To provide a molecular basis for designing better drugs targeting polymerases, African swine fever virus DNA Polymerase X (Pol X) was used as a model for the study. As the simplest DNA polymerase identified to date, Pol X belongs to the polymerase X family and is constituted of 174 amino acids. In this chemical reaction, metal-ion A (MeA) is a catalytic ion and decreases the pKa of 3′-OH, facilitating its attack on the α-phosphate of the incoming dNTP, and metal-ion B (MeB) stabilizes the dNTP-DNA-polymerase complex and increases the electrophilicity of the phosphorus center. To clearly understand the phosphodiester-bond-formation mechanism and the metal-ion catalysis of polymerases, we designed modified dNTP substrates with a chiral α-phosphorus center (α-P center) using a single selenium atom, without affecting the overall and local structures, to explore the absolute configuration inversion and probe the mechanisms of the metal ion–oxygen interactions.

To capture the reaction at the post-polymerization state, we designed and applied the crystallization droplets containing dGTPαSe-Rp, DNA-II, and Pol X. Surprisingly, we found that in one asymmetric unit, there was one substrate complex and three product complexes, including two DNA duplexes with four enzyme molecules. In other words, in the unit cell, the phosphoryl transfer reaction took place in three product complexes, whereas the last one was trapped in a transition-like state, where the incoming dGTPαSe-Rp paired with 5′-dC of the template strand. In the substrate complex, though two Me2+ ions at the active center coordinated with the incoming dGTPαSe-Rp, the phosphoryl transfer reaction did not occur, indicated by the clear density gap between the primer 3′-OH and the substrate α-phosphorus. Interestingly, the unexpected transition-like state complex revealed the in-line attacking SN2 mechanism in the phosphoryl-transfer polymerization, where with the attacking of the 3′-OH on the α-P center, a new bond was formed and the pyrophosphate was left. To catalyze the reaction, two Me2+ ions coordinated with the 3′-OH and the incoming dGTPαSe-Rp, whereas MeA interacted with the 3′-OH and Se atom and brought them together for the bond formation. The distance (3.3 Å) between the 3′-OH and the α-P atom was shorter than the relaxed distance (4.1 Å) provided in the literature, indicating the readiness state of the nucleophile for attacking. On the basis of the local structure (the trigonal bipyramid-like geometry) and the transition-like state, the attacking 3′-OH formed the hydrogen bond with the substrate 5′-O (indicated by their 2.8 Å distance), which facilitated the 3′-OH attacking and the phosphodiester bond formation. When compared to the structure of the native product complex, the Se-modified product complex (formed from dGTPαSe-Rp) generated extra and strong electron density only for the Se atom on the P-center, revealing its Sp configuration and indicating the two-metal Se coordination.

>[4x]GGGMLTLIQGKKIVNHLRSRLAFEYNGQLIKILSKNIVAVGSLRREEKMLNDVDLLIIVPEKKLLKHVLPNIRIKGLSFSVKVCGERKCVLFIEWEKKTYQLDLFTALAEEKPYAIFHFTGPVSYLIRIRAALKKKNYKLNQYGLFKNQTLVPLKITTEKELIKELGFTYRIPKKRL Panoptes is a two-gene operon, optSE, wherein OptS is predicted to synthesize a nucleotide-derived second messenger and OptE is predicted to bind that signal and drive effector-mediated defence. Crystal structures show that OptS is a minimal CRISPR polymerase (mCpol) domain, a version of the polymerase domain found in type III CRISPR systems (Cas10). OptS constitutively synthesizes 2′,3′-c-di-AMP and other cyclic dinucleotides to hold OptE in an inactive state. During phage infection, Acb2 or similar immune evasion proteins are produced that sequester the OptS-derived signalling molecule, leading to a population of OptE that is no longer bound to cyclic dinucleotide and is free to become activated, in turn disrupting the bacterial membrane and resulting in phage defence.

To better understand the possible enzymatic function of the OptS protein, we expressed and purified an orthologue from Klebsiella pneumoniae KP67 (KpOptS) for in vitro biochemical and structural characterization. We determined the crystal structure of KpOptS, which was refined at a nominal resolution of 1.75 Å. The crystallographic asymmetric unit contained four copies of KpOptS, forming an apparent tetrameric complex or dimer of dimers. Minimal conformational and B-factor variation was observed across the protomers and superposition showed root mean square deviation (r.m.s.d.) values of roughly 0.3–0.4 Å, on average, between pairs. A second interface connecting the two dimers has around 500 Å2 of buried surface area. It is not clear if this second interface is sufficient to determine whether the tetrameric complex represents a true species or whether it is a feature of crystallization. Although KpOptS is a small protein (about 14 kDa) on the basis of primary amino acid sequence alone, size-exclusion chromatography supported the existence of a larger molecular weight species in solution (greater than a dimer). Mass photometry experiments showed that KpOptS can exist as a stable tetramer in solution at low protein concentration (around 58 kDa monodisperse population observed at a concentration of roughly 50 nM). Although different in quaternary structure and domain architecture, the protomeric unit of KpOptS aligns well with the palm domains of Cas10 (Csm1) from Thermococcus onnurineus and the GGDEF diguanylate cyclase PleD from Caulobacter crescentus (r.m.s.d. values of 3.86 Å and 2.39 Å, respectively)30,31. GGDEF proteins are defined by a conserved linear sequence motif (glycine–glycine–[aspartate/glutamate]–[aspartate/glutamate]–phenylalanine) that is nearly absent from the mCpol proteins Kp and VnOptS, yet they still retain the characteristic β-hairpin structure and positioning of an acidic residue into the active site.

>MGSSHHHHHHGSMYIAIDGDDVGRKITSSYLSNSEERLTYISNKLNDTTKKISKMLLSNGFEIIFQAADGVTAKTDNEVNLNFVFDKIKSYSFDEITFSAGVGANLREAYVALLNSKSNGKNMISIYKDIL[4x]> VESIIKTATDTVKSEINAELGVV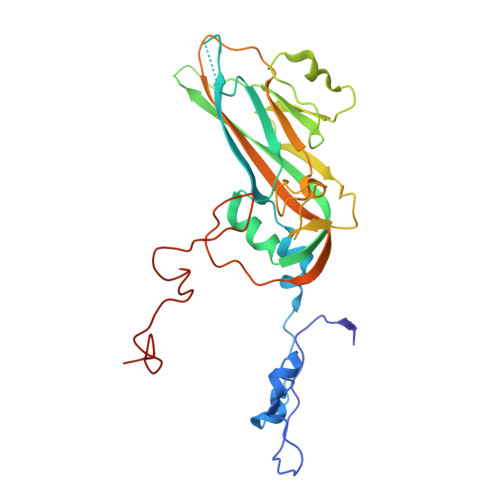PSLNAVETGATSNTEPEEAIQTRTVINQHGVSETLVENFLGRAALVSKKSFEYKNHASSSAGTHKNFFKWTINTKSFVQLRRKLELFTYLRFDAEITILTTVAVNGNNDSTYMGLPDLTLQAMFVPTGALTPKEQDSFHWQSGSNASVFFKISDPPARMTIPFMCINSAYSVFYDGFAGFEKNGLYGINPADTIGNLCVRIVNEHQPVGFTVTVRVYMKPKHIKAWAPRPPRTMPYMSIANANYKGRDTAPNTLNAIIGNRASVTTMPHNIVTT>GSHYNNAITPYLNKETGYQEMFQRVNTRIREFMINELKNHHNEDNVFMLAKNSGIEI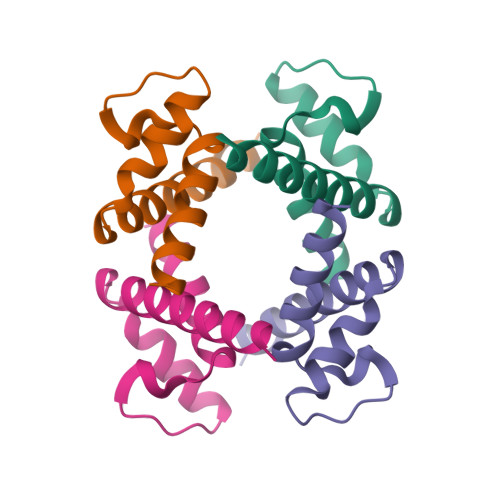AKIEEAPNAVLIPAFVLGELEVAFK[8x]>[3x]MFYSLMRESKIVIEYDGRGYHFDALSNYDASTSFQEFKTLRRTIHNRTNYADSIINAQDPSSISLAINFSTTLIESNFFDWMGFTREGNSLFLPRNTPNIEPIMFNMYIINHNNSCIYFENCYVSTVDFSLDKSIPILNVGIESGKFSEVSTFRDGYTITQGEVLPYSAPAVYTNSSPLPALISASMSFQQQCSWREDRNIFDINKIYTNKRAYVNEMNASATLAFYYVKRLVGDKFLNLDPETRTPLIIKNKYVSITFPLARISKRLNFSDLYQVEYDVIPTADSDPVEINFFGERK;>[6x]MRLPDPYTNPEYPGLGFESVNLVDNDPMIRDELPNGKVKEVKISAQYWGINISYPELFPDEYAFLDSRLLEYKRTGDYLDVLLPQYEAFRVRGDTKSVTIPAGQKGSQIILNTNGTLTGQPKAGDLFKLSTHPKVYKITNFSSSGNVWNISLYPDLFITTTGSEKPVFNGILFRTKLMNGDSFGSTLNNNGTYSGISLSLRESL;>[3x]MKKILDSAKNYLNTHDKLKTACLIALELPSSSGSAATYIYLTDYFRDVTYNGILYRSGKVKSISSHKQNRQLSIGSLSFTITGTAEDEVLKLVQNGVSFLDRGITIHQAIINEEGNILPVDPDTDGPLLFFRGRITGGGIKDNVNTSGIGTSVITWNCSNQFYDFDRVNGRYTDDASHRGLEVVNGTLQPSNGAKRPEYQEDYGFFHSNKSTTILAKYQVKEERYKLQSKKKLFGLSRSYSLKKYYETVTKEVDLDFNLAAKFIPVVYGVQKIPGIPIF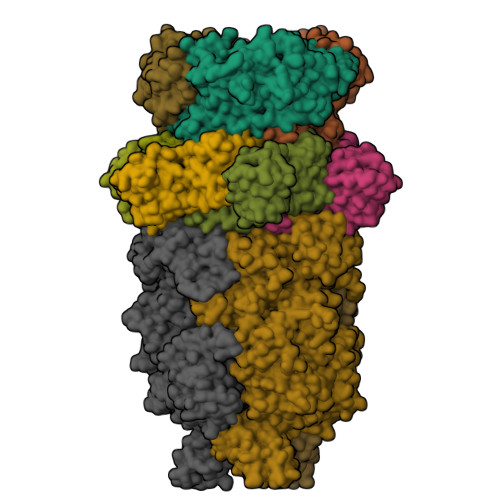ADTELNNPNIVYVVYAFAEGEIDGFLDFYIGDSPMICFDETDSDTRTCFGRKKIVGDTMHRLAAGTSTSQPSVHGQEYKYNDGNGDIRIWTFHGKPDQTAAQVLVDIAKKKGFYLQNQNGNGPEYWDSRYKLLDTAYAIVRFTINENRTEIPEISAEVQGKKVKVYNSDGTIKADKTSLNGIWQLMDYLTSDRYGADITLDQFPLQKVISEAKILDIIDESYQTSWQPYWRYVGWNDPLSENRQIVQLNTILDTSESVFKNVQGILESFGGAINNLSGEYRITVEKYSTNPLRINFLDTYGDLDLSDTTGRNKFNSVQASLVDPALSWKTNSITFYNSKFKEQDKGLDKKLQLSFANITNYYTARSYADRELKKSRYSRTLSFSVPYKFIGIEPNDPIAFTYERYGWKDKFFLVDEVENTRDGKINLVLQEYGEDVFINSEQVDNSGNDIPDISNNVLPPRDFKYTPTPGGVVGAIGKNGELSWLPSLTNNVVYYSIAHSGHVNPYIVQQLENNPNERMIQEIIGEPAGLAIFELRAVDINGRRSSPVTLSVDLNSAKNLSVVSNFRVVNTASGDVTEFVGPDVKLAWDKIPEEEIIPEIYYTLEIYDSQDRMLRSVRIEDVYTYDYLLTYNKADFALLNSGALGINRKLRFRIRAEGENGEQSVGWATI4-[(4R)-7-methyl-2,5-bis(oxidanylidene)-1-[3-(trifluoromethyl)phenyl]-3,4,6,8-tetrahydropyrimido[4,5-d]pyridazin-4-yl]benzenecarbonitrile 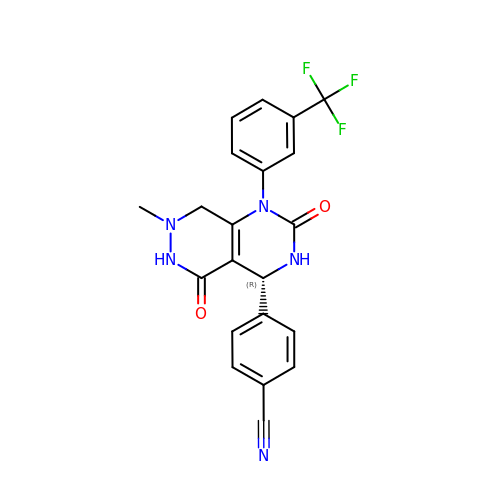| C21 H16 F3 N5 O2 | UPNMBPLODWPJQQ-GOSISDBHSA-N> PAPTVNTHFGKLRGARVPLPSEILGPVDQYLGVPYAAPPIGEKRFLPPEPPPSWSGIRNATHFPPVCPQNIHTAVPEVMLPVWFTANLDIVATYIQEPNEDCLYLNVYVPTEDGSGAKKQGEDLADNDGDEDEDIRDSGAKPVMVYIHGGSYMEGTGNMIDGSVLASYGNVIVITLNYRVGVLGFLSTGDQAAKGNYGLLDQIQALRWVSENIAFFGGDPRRITVFGSGIGASCVSLLTLSHHSEGLFQRAIIQSGSALSSWAVNYQPVKYTSLLADKVGCNVLDTVDMVDCLRQKSAKELVEQDIQPARYHVAFGPVIDGDVIPDDPEILMEQGEFLNYDIMLGVNQGEGLKFVEGVVDPEDGVSGTDFDYSVSNF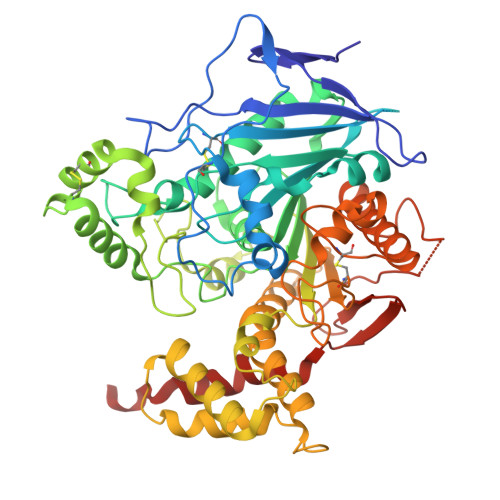VDNLYGYPEGKDTLRETIKFMYTDWADRDNPETRRKTLVALFTDHQWVEPSVVTADLHARYGSPTYFYAFYHHCQSLMKPAWSDAAHGDEVPYVFGVPMVGPTDLFPCNFSKNDVMLSAVVMTYWTNFAKTGDPNKPVPQDTKFIHTKANRFEEVAWSKYNPRDQLYLHIGLKPRVRDHYRATKVAFWKHLVPHLYNLHDMF2,2'-ethane-1,2-diylbis{5-[(sulfanylmethyl)amino]benzenesulfonic acid} | C16 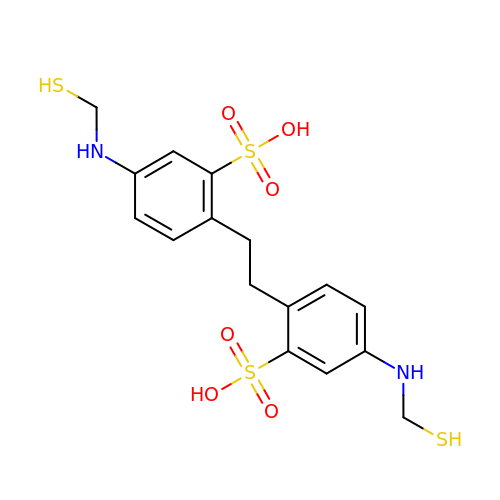H20 N2 O6 S4 | LJEHNCSYWIAXRX-UHFFFAOYSA-N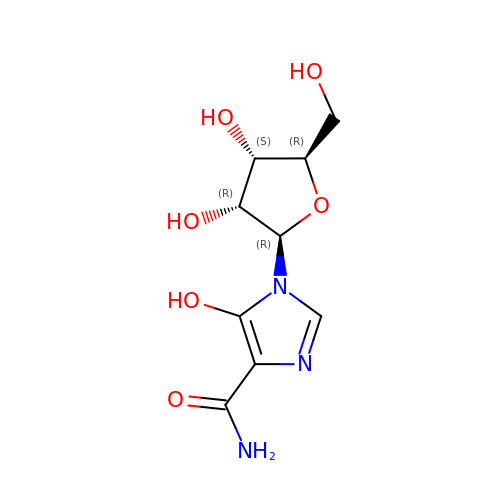5-hydroxy-1-(beta-D-ribofuranosyl)-1H-imidazole-4-carboxamide | C9 H13 N3 O6 | HZQDCMWJEBCWBR-UUOKFMHZSA-N>[4x]MGSSHHHHHHSSGLVPRGSMESGFTSK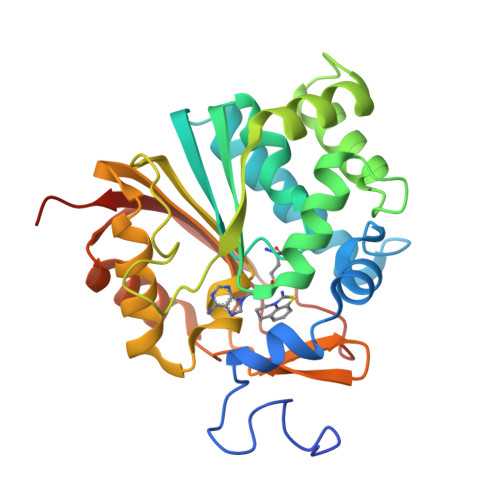DTYLSHFNPRDYLEKYYKFGSRHSAESQILKHLLKNLFKIFCLDGVKGDLLIDIGSGPTIYQLLSACESFKEIVVTDYSDQNLQELEKWLKAAPAAFDWSPVVTYVCDLEGNRVKGPEKEEKLRQAVKQVLKCDVTQSQPLGAVPLPPADCVLSTLCLDAACPDLPTYCRALRNLGSLLKPGGFLVIMDALKSSYYMIGEQKFSSLPLGREAVEAAVKEAGYTIEWFEVISQSYSSTMANNEGLFSLVARKLSRPL> DVQPETCRPSAASGNYFPQYPEYAIETARLRTFEAWPRNLKQKPHQLAEAGFFYTGVGDRVRCFSCGGGLMDWNDNDEPWE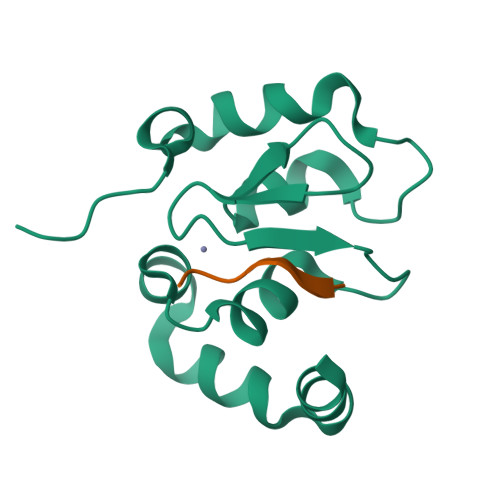QHALWLSQCRFVKLMKGQLYIDTVAAKPVLAEEKEESTSIGGD;> AIAYFIPDQA> MLDKIELFILDMDGTFYLDDSLLPGSLEFLETLKEKNKRFVFFTNNSSLGAQDYVRKLRNMGVDV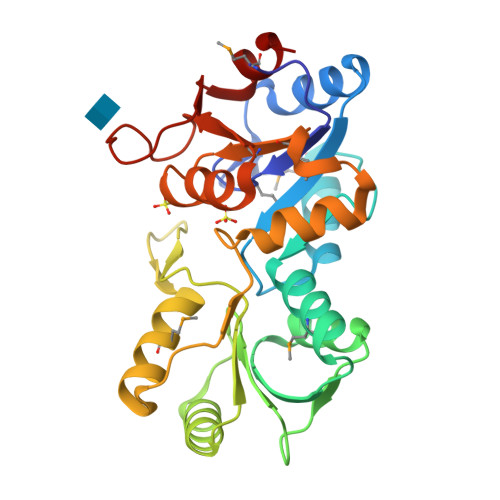PDDAVVTSGEITAEHMLKRFGRCRIFLLGTPQLKKVFEAYGHVIDEENPDFVVLGFDKTLTYERLKKACILLRKGKFYIATHPDINCPSKEGPVPDAGSIMAAIEASTGRKPDLIAGKPNPLVVDVISEKFGVPKERMAMVGDRLYTDVKLGKNAGIVSILVLTGETTPEDLERAETKPDFVFKNLGE Trypanothione reductase (TR) is a suitable target for drug discovery approaches against leishmaniasis, although the identification of potent inhibitors is still challenging. TR structure from different protozoan parasites has been extensively characterized by crystallography, showing that all key residues are conserved. This homodimeric flavoenzyme possesses four cavities binding two nicotinamide adenine dinucleotide phosphate hydrogen (NADPH) and two trypanothione molecules. Each NADPH cavity is separated from the trypanothione active site by a flavin adenine dinucleotide (FAD) cofactor allowing the transfer of two electrons by the participation of two catalytic cysteines (C52 and C57) which, together with H461′, E466′, and E467′ of the γ-Glu site, form the catalytic machinery. The active site features a hydrophobic cleft, named mepacrine binding site (MBS) after the crystal structure with the mepacrine inhibitor was solved.

To validate the predicted binding mode for further rational structure-based drug design and ligand optimization, the structures of TbTR with the most promising compounds 9, 10, and 14 were determined by X-ray crystallography. Additionally, with an eye to ligand efficiency, the p-fluorophenyl group in B of 5, 8, and 10 was removed while keeping in A the diClBn or the phenylpropane, leading to 12, 13, and 14, respectively. Quaternization of the piperazine promotes improvement in IC50 values compared to that of 5 (IC50 = 54.6 μM) by about 3-fold for 9 (IC50 = 20.5 μM), 42-fold for 10 (IC50 = 1.31 μM), and 23-fold for 14 (IC50 = 2.35 μM). However, this improvement does not seem to relate to the interaction between the positively charged ammonium and the protein but as shown in the solved structures, rather to the larger inhibitor structures, more efficiently occupying the binding pocket. The densities observed inside the trypanothione pocket for both TR dimers provided well-defined results for some portions of the compounds, namely, the ethyl-p-fluorophenyl and furan moieties, indicating that these common portions anchor 9, 10, and 14 to the Z-site by van der Waals and electrostatic interactions, as previously observed for fragment. From the interaction network, it is clear that the furan and the ethyl-p-fluorophenyl groups anchor 9, 10, and 14 to the Z-site, consistently with the binding of the initial fragments. It is also evident that the dichlorobenzyl group—when present—protrudes toward the MBS together with the phenylpropyl moiety, making a T-shaped π-stacking interaction with W21. Despite the presence of the bulkier side chains of M406 and Y106 in hGR (replacing the smaller L399 and A102 in TbTR), it seems that the binding of 10 and 14 toward hGR is not fully hampered. No clear correlation between the enzymatic and cellular activity could be delineated for the series, though the lowest EC50 value was obtained for 14 (EC50 = 8.98 μM), which is at the same time the second-best TR inhibitor (KiTR = 0.8 μM).

> SHMSKAFDLVVIGAGSGGLEAGWNAATLYGKRVAVVDVQTSHGPPFYAALGGTCVNVGCVPKKLMVTGAQYMDHLRESAGFGWEFDGSSVKANWKKLIAAKNEAVLDINKSYEGMFNDTEGLDFFLGWGSLESKNVVVVRETADPKSAVKERLQADHILLATGSWPQMPAIPGIEHCISSNEAFYLPEPPRRVLTVGGGFISVEFAGIFNAYKPPGGKVTLCYRNNLILRGFDETIREEVTKQLTANGIEIMTNENPAKVSLNTDGSKHVTFESGKTLDVDVVMMAIGRIPRTNDLQLGNVGVKLTPKGGVQVDEFSRTNVPNIYAIGDITDRLMLTPVAINEGAALVDTVFGNKPRKTDHTRVASAVFSIPPIGTCGLIEEVAAKEFEKVAVYMSSFTPLMHNISGSKYKKFVAKIVTNHSDGTVLGVHLLGDGAPEIIQAVGVCLRLNAKISDFYNTIGVHPTSAEELCSMRTPSYYYVKGEKMEKLPDSNLD;>[2x]SHMSKAFDLVVIGAGSGGLEAGWNAATLYGKRVAVVDVQTSHGPPFYAALGGTCVNVGCVPKKLMVTGAQYMDHLRESAGFGWEFDGSSVKANWKKLIAAKNEAVLDINKSYEGMFNDTEGLDFFLGWGSLESKNVVVVRETADPKSAVKERLQADHILLATGSWPQMPAIPGIEHCISSNEAFYLPEPPRRVLTVGGGFISVEFAGIFNAYKPPGGKVTLCYRNNLILRGFDETIREEVTKQLTANGIEIMTNENPAKVSLNTDGSKHVTFESGKTLDVDVVMMAIGRIPRTNDLQLGNVGVKLTPKGGVQVDEFSRTNVPNIYAIGDITDRLMLTPVAINEGAALVDTVFGNKPRKTDHTRVASAVFSIPPIGTCGLIEEVAAKEFEKVAVYMSSFTPLMHNISGSKYKKFVAKIVTNHSDGTVLGVHLLGDGAPEIIQAVGVCLRLNAKISDFYNTIGVHPTSAEELCSMRTPSYYYVKGEKMEKLPDSNL;> GSHMSKAFDLVVIGAGSGGLEAGWNAATLYGKRVAVVDVQTSHGPPFYAALGGTCVNVGCVPKKLMVTGAQYMDHLRESAGFGWEFDGSSVKANWKKLIAAKNEAVLDINKSYEGMFNDTEGLDFFLGWGSLESKNVVVVRETADPKSAVKERLQADHILLATGSWPQMPAIPGIEHCISSNEAFYLPEPPRRVLTVGGGFISVEFAGIFNAYKPPGGKVTLCYRNNLILRGFDETIREEVTKQLTANGIEIMTNENPAKVSLNTDGSKHVTFESGKTLDVDVVMMAIGRIPRTNDLQLGNVGVKLTPKGGVQVDEFSRTNVPNIYAIGDITDRLMLTPVAINEGAALVDTVFGNKPRKTDHTRVASAVFSIPPIGTCGLIEEVAAKEFEKVAVYMSSFTPLMHNISGSKYKKFVAKIVTNHSDGTVLGVHLLGDGAPEIIQAVGVCLRLNAKISDFYNTIGVHPTSAEELCSMRTPSYYYVKGEKMEKLPDSNL> MENF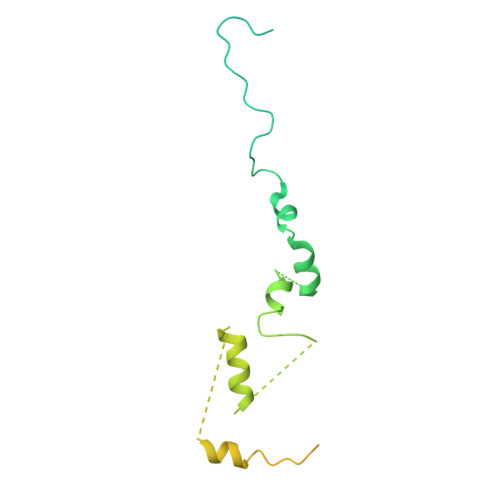TALFGAQTDPPPPPSALGFGPGKPPPPPPPPPGGGPGAAPPSTATSAPAGADKSTAGSGPFYLMRELPGSTELTGSTNLITHYNLEQAYNKFCGKKVKEKLSNFLPDLPGMIDLPGSHDNSSLRSLIEKPPILGGSFNPITGTMLSGFRLHTGPLPEQCRLMHIQPPKKKNKHKHKQSRTQDPVPPETPSDSDHKKKKKKKEEDPERKRKKKEKKKKKNRHSPDHPGMGSSQASSS>GPKTLKFMTASSPLSPKDPNEKLILQRLEKETGVHIDWTNYQSDFAEKRNLDISSGDLPDAIHNDGASDVDLMNWAKKGVIIPVEDLIDKYMPNLKKILDEKPEYKALMTAPDGHIYSFPWIEELGDGKESIHSVNDMAWINKDWLKKLGLEMPKTTDDLIKVLEAFKNGDPNGNGEAAAIPFSFISGNGNEDFKFLFAAFGIGDNDDHLVVGNDGKVDFTADNDNYKEGVKFIRQLQEKGLIDKEAFEHDWNSYIAKGHDQKFGVYFTWDKNNVTGSNESYDVLPVLAGPSGQKHVARTNGMGFARDKMVITSVNKNLELTAKWIDAQYAPLQSVQNNWGTYGDDKQQNIFELDQASNSLKHLPLNGTAPAELRQKTEVGGPLAILDSYYGKVTTMPDDAKWRLDLIKEYYVPYMSNVNNYPRVFMTQEDLDKIAHIEADMNDYIYRKRAEWIVNGNIDTEWDDYKKELEKYGLS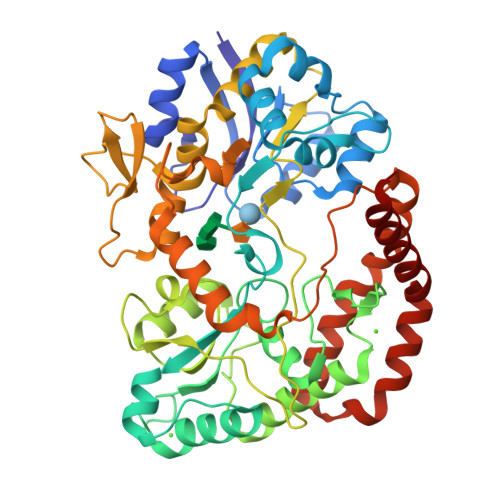DYLAIKQKYYDQYQANKN[2x]> MSEFLTPERTVYDSGVQFLRPKSLDEFIGQENVKKKLSLALEAAKMRGEVLDHVLLAGPPGLGRTTLAHIIASELQTNIHVTSGPVLVKQGDMAAILTS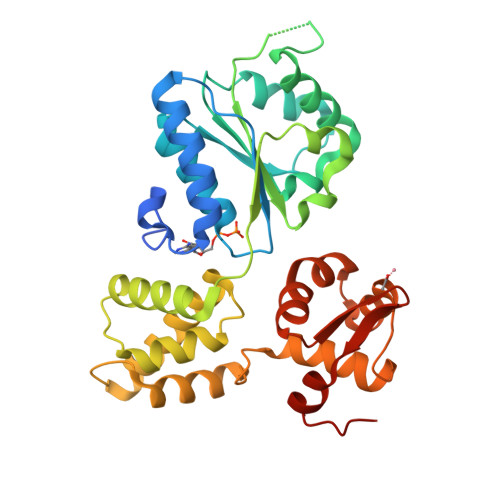LERGDVLFIDEIHRLNKAVEELLYSAIEDFQIDIMIGKGPSAKSIRIDIQPFTLVGATTRSGLLSSPLRSRFGIILELDFYTVKELKEIIKRAASLMDVEIEDAAAEMIAKRSRGTPRIAIRLTKRVRDMLTVVKADRINTDIVLKTMEVLNIDDEGLDEFDRKILKTIIEIYRGGPVGLNALAASLGVEADTLSEVYEPYLLQAGFLARTPRGRIVTEKAYKHLKYEVPENRLF> MSEFRIHHDVNELLSLLRVHGGDGAEVYIDLLQKNRTPYVTTTVSAHSAKVKIAEFSRTPEDFLKKYDELKSKNTRNLDPLVYLLSKLTEDKETLQYLQQNAKERAELAAAAVGSSTTSINVPAAASKISMQELEELRKQLGSVATGSTLQQSLELKRKMLRDKQNKKNSGQHLPIFPAWVYERPALIGDFLIGAGISTDTALPIGTLPLASQESAVVEDLLYVLVGVDGRYVSAQPLAGRQSRTFLVDPNLDLSIRELVHRILPVAASYSAVTRFIEEKSSFEYGQVNHALAAAMRTLVKEHLILVSQLEQLHRQGLLSLQKLWFYIQPAMRTMDILASLATSVDKGECLGGSTLSLLHDRSFSYTGDSQAQELCLYLTKAASAPYFEVLEKWIYRGIIHDPYSEFMVEEHELRKERIQEDYNDKYWDQRYTIVQQQIPSFLQKMADKILSTGKYLNVVRECGHDVTCPVAKEIIYTLKERAYVEQIEKAFNYASKVLLDFLMEEKELVAHLRSIKRYFLMDQGDFFVHFMDLAEEELRKPVEDITPPRLEALLELALRMSTANTDPFKDDLKIDLMPHDLITQLLRVLAIETKQEKAMAHADPTELALSGLEAFSFDYIVKWPLSLIINRKALTRYQMLFRHMFYCKHVERQLCSVWISNKTAKQHSLHSAQWFAGAFTLRQRMLNFVQNIQYYMMFEVMEPTWHILEKNLKSASNIDDVLGHHTGFLDTCLKDCMLTNPELLKVFSKLMSVCVMFTNCMQKFTQSMKLDGELGGQTLEHSTVLGLPAGAEERARKELARKHLAEHADTVQLVSGFEATINKFDKNFSAHLLDLLARLSIYSTSDCEHGMASVISRLDFNGFYTERLERLSAERSQKATPQVPVLRGPPAPAPRVAVTAQ;>MATPDQKSPNVLLQNLCCRILGRSEADVAQQFQYAVRVIGSNFAPTVERDEFLVAEKIKKELIRQRREADAALFSELHRKLHSQGVLKNKWSILYLLLSLSEDPRRQPSKVSSYATLFAQALPRDAHSTPYYYARPQTLPLSYQDRSAQSAQSSGSVGSSGISSIGLCALSGPAPAPQSLLPGQSNQAPGVGDCLRQQLGSRLAWTLTANQPSSQATTSKGVPSAVSRNMTRSRREGDTGGTMEITEAALVRDILYVFQGIDGKNIKMNNTENCYKVEGKANLSRSLRDTAVRLSELGWLHNKIRRYTDQRSLDRSFGLVGQSFCAALHQELREYYRLLSVLHSQLQLEDDQGVNLGLESSLTLRRLLVWTYDPKIRLKTLAALVDHCQGRKGGELASAVHAYTKTGDPYMRSLVQHILSLVSHPVLSFLYRWIYDGELEDTYHEFFVASDPTVKTDRLWHDKYTLRKSMIPSFMTMDQSRKVLLIGKSINFLHQVCHDQTPTTKMIAVTKSAESPQDAADLFTDLENAFQGKIDAAYFETSKYLLDVLNKKYSLLDHMQAMRRYLLLGQGDFIRHLMDLLKPELVRPATTLYQHNLTGILETAVRATNAQFDSPEILRRLDVRLLEVSPGDTGWDVFSLDYHVDGPIATVFTRECMSHYLRVFNFLWRAKRMEYILTDIRKGHMCNAKLLRNMPEFSGVLHQCHILASEMVHFIHQMQYYITFEVLECSWDELWNKVQQAQDLDHIIAAHEVFLDTIISRCLLDSDSRALLNQLRAVFDQIIELQNAQDAIYRAALEELQRRLQFEEKKKQREIEGQWGVTAAEEEEENKRIGEFKESIPKMCSQLRILTHFYQGIVQQFLVLLTTSSDESLRFLSFRLDFNEHYKAREPRLRVSLGTRGRRSSHT[2x];>[2x]MIHELLLALSGYPGSIFTWNKRSGLQVSQDFPFLHPSETSVLNRLCRLGTDYIRFTEFIEQYTGHVQQQDHHPSQQGQGGLHGIYLRAFCTGLDSVLQPYRQALLDLEQEFLGDPHLSISHVNYFLDQFQLLFPSVMVVVEQIKSQKIHGCQILETVYKHSCGGLPPVRSALEKILAVCHGVMYKQLSAWMLHGLLLDQHEEFFIKQGPSSGNVSAQPEEDEEDLGIGGLTGKQLRELQDLRLIEEENMLAPSLKQFSLRVEILPSYIPVRVAEKILFVGESVQMFENQNVNLTRKGSILKNQEDTFAAELHRLKQQPLFSLVDFEQVVDRIRSTVAEHLWKLMVEESDLLGQLKIIKDFYLLGRGELFQAFIDTAQHMLKTPPTAVTEHDVNVAFQQSAHKVLLDDDNLLPLLHLTIEYHGKEHKADATQAREGPSRETSPREAPASGWAALGLSYKVQWPLHILFTPAVLEKYNVVFKYLLSVRRVQAELQHCWALQMQRKHLKSNQTDAIKWRLRNHMAFLVDNLQYYLQVDVLESQFSQLLHQINSTRDFESIRLAHDHFLSNLLAQSFILLKPVFHCLNEILDLCHSFCSLVSQNLGPLDERGAAQLSILVKGFSRQSSLLFKILSSVRNHQINSDLAQLLLRLDYNKYYTQAGGTLGSFGM;>[2x]MARHGPPWSRLDAQQERDVRELVRGVAGLQDEADPNFQLALNFAWSNFRFHRFLDVNSHKIEKTIEGIYEKFVIHSDLSKAASWKRLTEEFLNAPLPSIKEIKTDAHYSILSLLLCLSDSPSNSSYVETPRNKEVEKKDDFDWGKYLMEDEEMDIGPYMDTPNWSEESEEENDQQPLSREDSGIQVDRTPLEEQDQNRKLDPCISWKDEPDDRSWLEHHVVHQYWTARPSQFPHSLHLHSNLAAVWDQHLYSSDPLYVPDDRVLVTETQVIRETLWLLSGVKKLFIFQLIDGKVTVRNNIIVTHLTHSCLRSVLEQIAAYGQVVFRLQEFIDEVMGHSSESMLPGSGSVPKKSTEAPFRTYQAFMWALYKYFISFKEELAEIEKCIINNDTTITLAIVVDKLAPRLSQLKVLHKVFSTGVAEVPPDTRNVVRASHLLNTLYKAILEYDNVGEASEQTVSLLFSLWVETVRPYLQTVDEWIVHGHLWDGAREFIIQRNKNVPVNHRDFWYATYTLYSVSEKTENEEKMSDNASASSGSDQGPSSRQHTMVSFLKPVLKQIIMAGKSMQLLKNLQCAESTTCQAGARDAERKSLYTLFLESVQSRLRHGEDSTPQVLTEQQATKENLMKMQSIAESHLELDDVHDPLLAINFARMYLEQSDFHEKFAGGDVCVDRSSESVTCQTFELTLRSCLYPHIDKQYLDCCGNLMQTLKKDYRLVEYLQAMRNFFLMEGGDTMYDFYTSIFDKIREKETWQNVSFLNVQLQEAVGQRYPEDSSRLSISFENVDTAKKKLPVHILDGLTLSYKVPWPVDIVISLECQKIYNQVFLLLLQIKWAKYSLDVLLFGELVSTAEKPRLKEGLIHEQDTVAQFGPQKEPVRQQIHRMFLLRVKLMHFVNSLHNYIMTRILHSTGLEFQHQVEEAKDLDQLIKIHYRYLSTIHDRCLLREKVSFVKEAIMKVLNLALMFADGWQAGLGTWRMESIEKMESDFKNCHMFLVTILNKAVCRGSFPHLESLALSLMAGMEQS;> MASITQLFDDLCEALLPAAKTHLGQRSVNRKRAKRSLKKVAYNALFTNLFQDETQQLQPDMSKLPARNKILMLSFDLRVGGLGPKADRLEELVEELEAAPCCPLLEVGSVLDLLVQLAGSGPPQVLPRKRDYFLNNKHVGRNVPYSGYDCDDLSVFEMDVQSLISREECLCHSMIQETLQVMEAAPGTGLPTVGLFSFGDPCGDRFERDTRVSLFGALVHSRTYDMDVRLGLPPVPDNADLSGLAIKVPPSVDQWEDEGFQSASNLTPDSQSEPSVTPDVDLWEAALTYEASKRRCWERVGCPPGHREEPYLTEAGRDAFDKFCRLHQGELQLLAGGVLQAPQPVLVKECELVKDVLNVLIGVVSATFSLCQPAQAFVVKRGVHVSGASPESISSLLSEVAEYGTCYTRLSHFSLQPVLDSLYSKGLVFQAFTSGLRRYLQYYRACVLSTPPTLSLLTIGFLFKKLGRQLRYLAELCGVGAVLPGTCGGGPRAAFPTGVKLLSYLYQEALHNCSNEHYPVLLSLLKTSCEPYTRFIHDWVYSGVFRDAYGEFMIQVNHEYLSFRDKLYWTHGYVLISKEVEDCVPVFLKHIAHDIYVCGKTINLLKLCCPRHYLCWSDVPVPRISVIFSLEELKEIEKDCAVYVGRMERVARHSSVSKEEKELRMEIAKQELIAHAREAASRVLSALSDRQMSERMALDARKREQFQRLKEQFVKDQERRQAARQEELDDDFSYARELRDRERRLKSLEEELERKARQALVDHYSKLSAEAARREQKALWRIQRHRLESARLRFLLEDEKHIQEMLKAVSEAHQPQEPPDVLLSVHPQVTSPGPEHPEGGQGCDSGSAEQHSPAWDGWNRPGLLTPQPLKPLAVGAGGRGLQQAEGARPFSDSLSIGDFLPVGPGAEPSVQTGMVPLLEVALQTINLDLPPSAPGEAPAAASTQPSRPQEYDFSTVLRPAVATSPAPGPLQAAECSLGSSGLQLWEDSCGKMDACGSASRETLLPSHPPRRAALEEGSSQPTERLFGQVSGGGLPTGDYASEIAPTRPRWNTHGHVSDASIRVGENVSDVAPTQPRWNTHGHVSNASISLGESVSDVAPTRPRWNIHGHVSNASIRVGENVSDVAPTRPRWNTHGHVSNASIRVGENVSDVAPTRPRWNTHGHVSDASISLGESVSDMAPARPRWNTHGHVSDASISLGESVSDMAPTRPRWNTHGHVSDTSIRVGENVSDVAPIRSRCNTHGHVSDASISLGEPVSDVVSTRPRWNTHVPIPPPHMVLGALSPEAEPNTPRPQQSPPGHTSQSALSLGAQSTVLDCGPRLPVEVGPSLSSPSSGCGEGSISVGENVSDVAPTQPWWPNTPGDSVSEELGPGRSGDTEDLSPNWPLNSQEDTAAQSSPGRGEEAEASAAEAQGGEQAYLAGLAGQYHLERYPDSYESMSEPPIAHLLRPVLPRAFAFPVDPQVQSAADETAVQLSELLTLPVLMKRSITAPLAAHISLVNKAAVDYFFVELHLEAHYEALRHFLLMEDGEFAQSLSDLLFEKLGAGQTPGELLNPLVLNSVLSKALQCSLHGDTPHASNLSLALKYLPEVFAPNAPDVLSCLELRYKVDWPLNIVITEGCVSKYSGVFSFLLQLKLMMWALKDVCFHLKRTALLSHMAGSVQFRQLQLFKHEMQHFVKVIQGYIANQILHVTWCEFRARLATVGDLEEIQRAHAEYLHKAVFRGLLTEKAAPVMNVIHSIFSLVLKFRSQLISQAWGPPGGPRGAEHPNFALMQQSYNTFKYYSHFLFKVVTKLVNRGYQPHLEDFLLRINFNNYYQDA;>[6x]MPREIITLQLGQCGNQIGFEFWKQLCAEHGISPE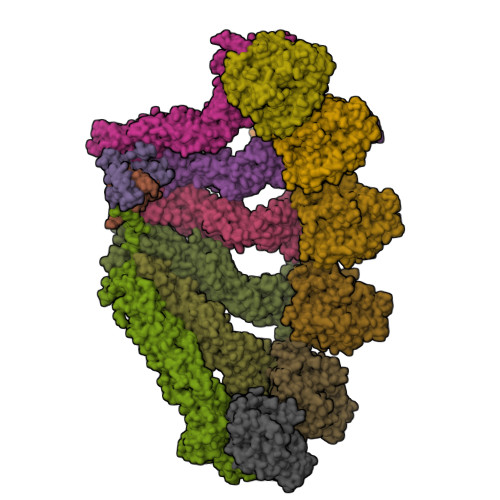GIVEEFATEGTDRKDVFFYQADDEHYIPRAVLLDLEPRVIHSILNSPYAKLYNPENIYLSEHGGGAGNNWASGFSQGEKIHEDIFDIIDREADGSDSLEGFVLCHSIAGGTGSGLGSYLLERLNDRYPKKLVQTYSVFPNQDEMSDVVVQPYNSLLTLKRLTQNADCVVVLDNTALNRIATDRLHIQNPSFSQINQLVSTIMSASTTTLRYPGYMNNDLIGLIASLIPTPRLHFLMTGYTPLTTDQSVASVRKTTVLDVMRRLLQPKNVMVSTGRDRQTNHCYIAILNIIQGEVDPTQVHKSLQRIRERKLANFIPWGPASIQVALSRKSPYLPSAHRVSGLMMANHTSISSLFERTCRQYDKLRKREAFLEQFRKEDMFKDNFDEMDTSREIVQQLIDEYHAATRPDYISWGTQEQ;>MASSSGAGAAAAAAAANLNAVRETMDVLLEISRILNTGLDMETLSICVRLCEQGINPEALSSVIKELRKATEALKAAENMTS[2x]> GAMGSRLYDRRSIFDAVAQSNCQELESLLPFLQRSKKRLTDSEFKDPETGKTCLLKAMLNLHNGQNDTIALLLDVARKTDSLKQFVNASYTDSYYKGQTALHIAIERRNMTLVTLLVENGADVQAAANGDFFKKTKGRPGFYFGELPLSLAACTNQLAIVKFLLQNSWQPADISARDSVGNTVLHALVEVADNTVDNTKFVTSMYNEILILG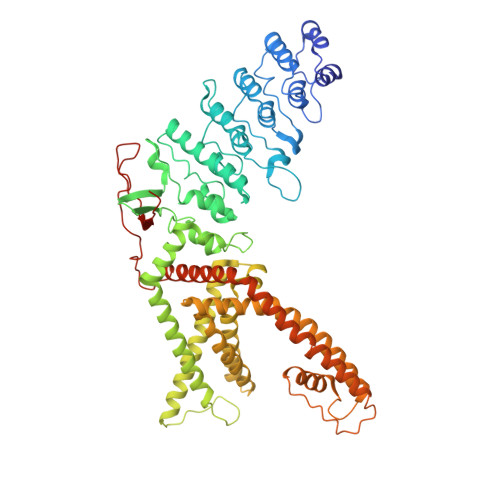AKLHPTLKLEEITNRKGLTPLALAASSGKIGVLAYILQREIHEPECRHLSRKFTEWAYGPVHSSLYDLSCIDTCEKNSVLEVIAYSSSETPNRHDMLLVEPLNRLLQDKWDRFVKRIFYFNFFVYCLYMIIFTAAAYYRPVEGLPPYKLKNTVGDYFRVTGEILSVSGGVYFFFRGIQYFLQRRPSLKSLFVDSYSEILFFVQSLFMLVSVVLYFSQRKEYVASMVFSLAMGWTNMLYYTRGFQQMGIYAVMIEKMILRDLCRFMFVYLVFLFGFSTAVVTLIEDGKYNSLYSTCLELFKFTIGMGDLEFTENYDFKAVFIILLLAYVILTYILLLNMLIALMGETVNKIAQESKNIWKLQRAITILDTEKSFLKCMRKAFRSGKLLQVGFTPDGKDDYRWCFRVDEVNWTTWNTNVGIINEDPG> GVFLADASANDAAKKLYKYLRLVYGNKILSGMMAHVAWNHDEADKIHVLTGKYPAINCYDFIHIAVPNQGSNGWINYNDITPVTEWADAGGI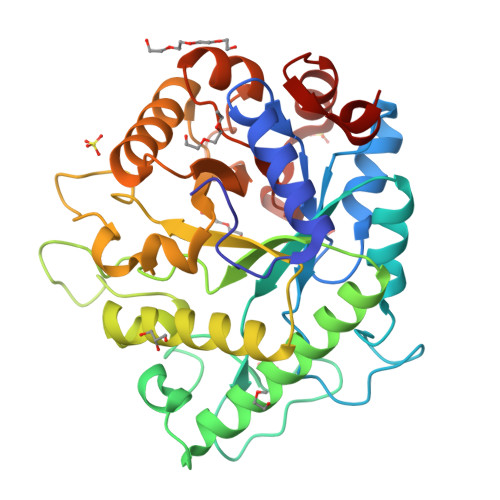VSLMWHFNVPQNENTTIGADGSGQGINSSQTTFKASHALVSGTWENKFFMEQMENVANVILKLQDAGIVALWRPFHEAAGNATLKSGANWGKAWFWWGEDGPDVYKQLWHTMFNYFSNKGIHNLIWEWTSQNYNGDSDIYNNDDDWYPGDAYVDIIGRDLYGTTAVQQYSEYSQLKGRYPSKMIALAECGVNNSTITADVEQAWNAGAKWLNFMPWYGESMPSDEWWTKVMNENVVITRDEINQN>[2x]MADPLTPAISDRICKHMNEDAASA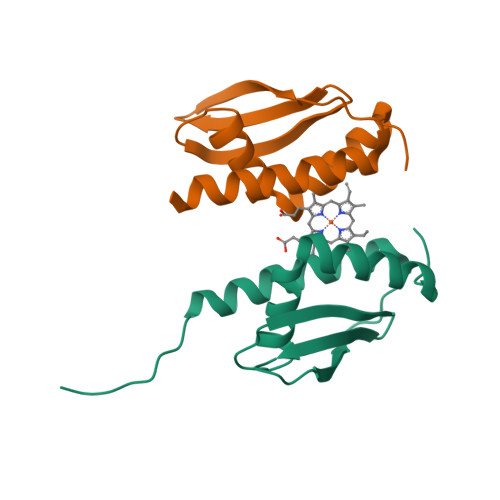IALYAQVFGQQTDVTMAQMQAIDPTGMDLVVESEGGSKTIRIEFEQPLKDSEDAHQVLIAMAKQARSVGKNSAENLYFQ> SKSKVDNQFYSVEVGDSTFTVLKRYQNLKPIGSGAQGIVCAAYDAVLDRNVAIKKLSRPFQNQTHAKRAYRELVLMKCVNHKNIISLLNVFTPQKTLEEFQDVYLVMELMDANLCQVIQMELDHERMSYLLYQMLCGIKHLHSAGIIHRDLKPSNIVVKSDCTLKILDFGLARTAGTSFMMTPYVVTRYYRAPEVILGMGYKENVDIWSVGCIMGEMVRHKILFPGRDYIDQWNKVIEQLGTPCPEFMKKLQP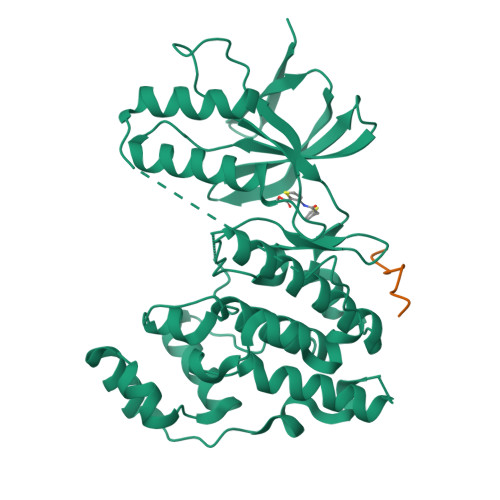TVRNYVENRPKYAGLTFPKLFPDSLFPADSEHNKLKASQARDLLSKMLVIDPAKRISVDDALQHPYINVWYDPAEVEAPPPQIYDKQLDEREHTIEEWKELIYKEVMNS;> PKRPTTLNLF>[4x]ATSDSNMLLNYVPVYVMLPLGVVNVDNVFEDPDGLKEQLLQLRAAGVDGVMVDVWWGIIELKGPKQYDWRAYRSLLQLVQECGLTLQAIMSFHQCGGNVGDIVNIPIPQWVLDIGESNHDIFYTNRSGTRNKEYLTVGVDNEPIFHGRTAIEIYSDYMKSFRENMSDFLESGLIIDIEVGLGPAGELRYPSYPQSQGWEFPGIGEFQCYDKYLKADFKAAVARAGHPEWELPDDAGKYNDV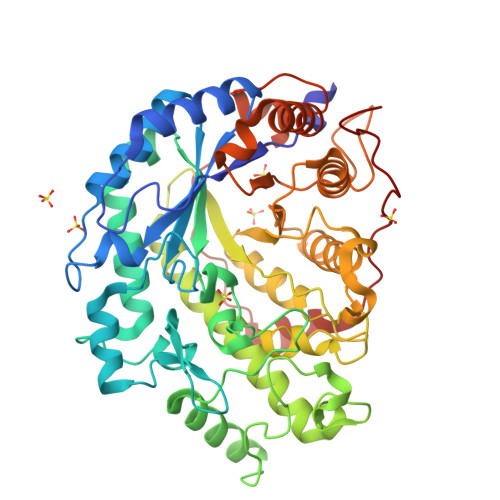PESTGFFKSNGTYVTEKGKFFLTWYSNKLLNHGDQILDEANKAFLGCKVKLAIKVSGIHWWYKVENHAAELTAGYYNLNDRDGYRPIARMLSRHHAILNFTCLEMRDSEQPSDAKSGPQELVQQVLSGGWREYIRVAGENALPRYDATAYNQIILNARPQGVNNNGPPKLSMFGVTYLRLSDDLLQKSNFNIFKKFVLKMHADQDYCANPQKYNHAITPLKPSAPKIPIEVLLEATKPTRPFPWLDETDMKVDG>MKTIRRYDVNEDRGHTGLVEAGDFYYLNYCVGNVGQDIESQINGAFDEMERRLALVGLTLDAVVQMDCLFRDVWNIPVMEKMIKERFNGRYPARKSIQTEFAHHGGPQGLLFQVDGVA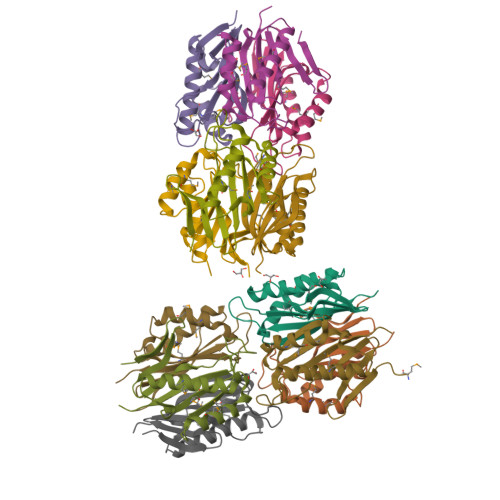YSKHISMT[12x]>GKLNIVTTFYPVYEFTKQVAGD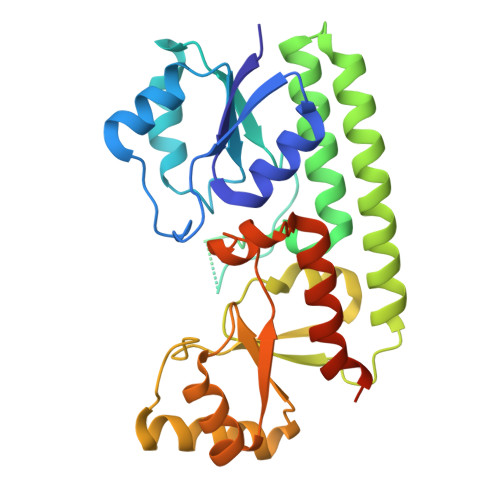TANVELLIGAGTEPHEYEPSAKAVAKIQDADTFVYENENMETWVPKLLDTLDKKKVKTIKATGDMLLLPGGEEEEGDHDHGEEGHHHEFDPHVWLSPVRAIKLVEHIRDSLSADYPDKKETFEKNAAAYIEKLQSLDKAYAEGLSQAKQKSFVTQHAAFNYLALDYGLKQVAISGLSPDAEPSAARLAELTEYVKKNKIAYIYFEENASQALANTLSKEAGVKTDVLNPLESLTEEDTKAGENYISVMEKNLKALKQTTDQEGPAIEPEKAEDTKTV[4x]>[12x]MDPVYVDIDADSAFLKALQRAYPMFEVEPRQVTPNDHANARAFSHLAIKLIEQEIDPDSTILDIGSAPARRMMSDRKYHCVCPMRSAEDPERLANYARKLASAAGKVLDRNISGKIGDLQAVMAVPDTETPTFCLHTDVSCRQRADVAIYQDVYAVHAPTSLYHQAIKGVRLAYWVGFDTTPFMYNAMAGAYPSYSTNWADEQVLKAKNIGLCSTDLTEGRRGKLSIMRGKKLEPCDRVLFSVGS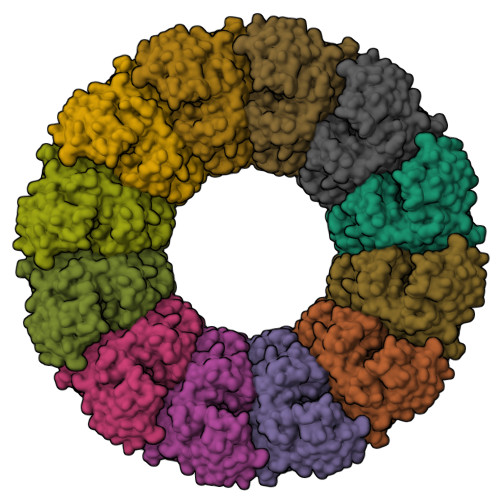TLYPESRKLLKSWHLPSVFHLKGKLSFTCRCDTVVSCEGYVVKRITMSPGLYGKTTGYAVTHHADGFLMCKTTDTVDGERVSFSVCTYVPATICDQMTGILATEVTPEDAQKLLVGLNQRIVVNGRTQRNTNTMKNYMIPVVAQAFSKWAKECRKDMEDEKLLGVRERTLTCCCLWAFKKQKTHTVYKRPDTQSIQKVQAEFDSFVVPSLWSSGLSIPLRTRIKWLL>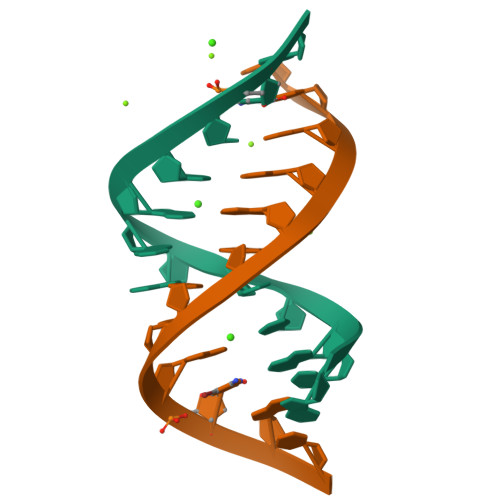 GCGUCAGGUCCG;> CGGAAGCAGCGC>[4x]MHDLRISLVQGSTRWHDPAG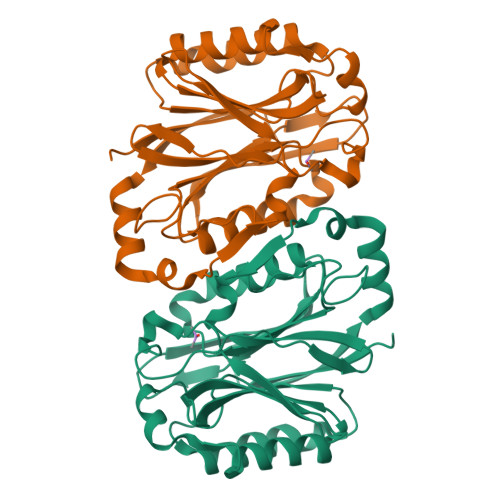NRDYYGALLEPLAGQSDLVILPETFTSGFSNEAIDKAEDMDGPTVAWIRTQAARLGAAITGSVQLRTEHGVFNRLLWATPDGALQYYDKRHLFRFGNEHLRYAAGRERLCVEWKGWRINPQVCYDLRFPVFCRNRFDVERPGQLDFDLQLFVANWPSARAYAWKTLLRARAIENLCFVAAVNRVGVDGNQLHYAGDSAVIDFLGQPQVEIREQEQVVTTTISAAALAEHRARFPAMLDGDSFVLGE> SLMSVDPNYTEMEGKVREATNNEPWGAS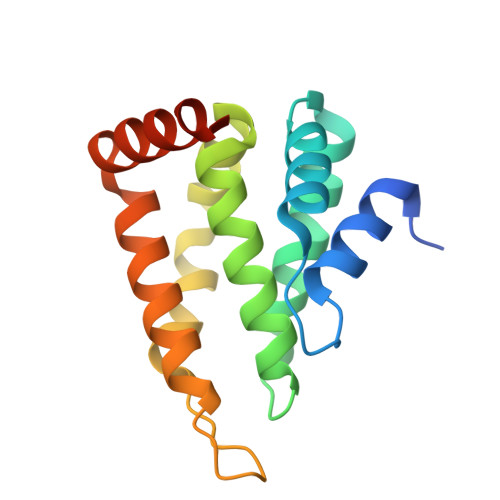STLMDQISQGTYNFREREEILSMIFRRFTEKAGSEWRQIYKALQLLDYLIKHGSERFIDDTRNSINLIRILETFHYIDSQGRDQGINVRTRVKALIELLSDDNKIRAERKKARETAKKYKGV> MTENILRKSDEEIQKEITARVKALESMLIEQGILTTSMIDRMAEIYENEVGPHLGAKVVVKAWTD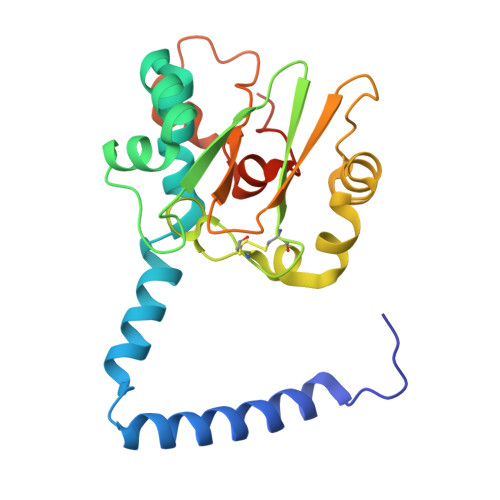PEFKKRLLADGTEACKELGIGGLQGEDMMWVENTDEVHHVVVCTLCSCYPWPVLGLPPNWFKEPQYRSRVVREPRQLLKEEFGFEVPPSKEIKVWDASSEMRFVVLPQRPAGTDGWSEEELATLVTRESMIGVEPAKAVAHHHHHH>[2x]MVNYE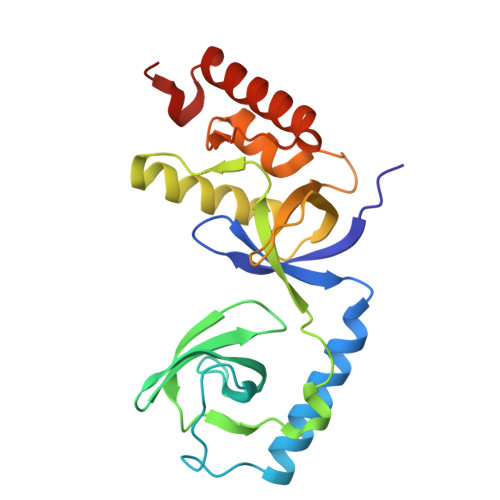NVIVTEITETLTFFAQSVESGSKLESLMSKLHADFQSNPPIAGSYTPKRGDLVAAQFTLDNQWYRAKVERVQGSNATVLYIDYGNKETLPTNRLAALPPAFSSEKPYATEYALALVALPTDNEDKEEALRAFSEDVLNHKVQLNVELKVTGSPNLATLRDPTTKVDFGKQLVAEGLVLAEQRGERKLKELVDQYKAAQEAARVAHLAIWKYGD>MPSYLSPGVYVEEVASGSRPIEGVGIEGVGTSVAAFVGLAPTGPLNEPTLVTNWTQYVAAFGDFTGGYYLAHSVYGFFNNGGSAAYVVRVGGSAEDAAADGSVNGAAAPAAVTGSTAKALPAAEPKQLGTFAVTATAAGQSGPLTVEVADPEGEGPAERFKLIVKDGDKPVETFDVSAKKGNRSYVVTQVKERSKLITVTEAAPSAQLVRPENQSLTLPAPPSAAPAVPAGQAESAHPGPAQYLGDSSDRTGFGGLEAIDEISMVAVPDLMAAYQRGAIDLEAVKAVQLGLIAHCELMGDRVAIIDPPPNQNARQIRVWRQETAGYDSKYAALYYPWIKSFDPATGQSRLVPPSGHVAGIWARNDSERGVHKAPANEVVRGAVDLELQITRGEQDLLNPIGVNCIRSFPGRGIRVWGARTLSSDPAWRYLNIRRYFNYLEESILIGTQWVVFEPNDHNLWARIRRNVSAFLVNEWRNGALFGQSPDQAYYVKCDEETNPPESVDLGRVVCEIGIAPVKPAEFVIFRLAQFSSGGGELDE[24x];>[24x]MSLPKPEDVLVAPNFGIQIDGVMVEYLNSVSNLQIEQDVIRYQQNQGTTGRNNVTLMPGVAKDG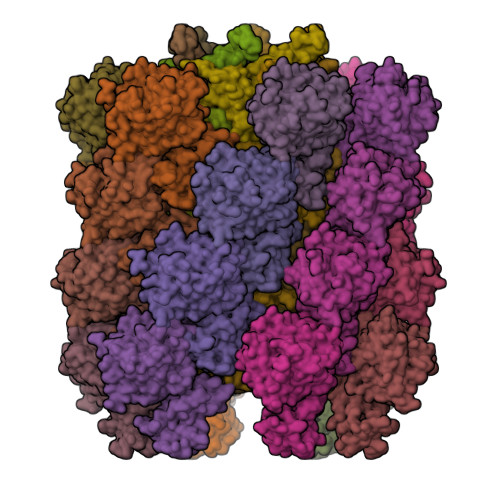SVQVERGMSQSSVFTQWINDSMAGRMATARKNATIIVMDYEDNPVKRWNLRNAWCSKVVAGTLKAGDTNALTETITIVFEELVVE>VRSFIYEPFQIPSGSMMPTLLIGDFILVEKFAYGIKDPIYQKTLIETGHPKRGDIVVFKYPEDPKLDYIKRAVGLPGDKVTYDPVSKELTIQPGCSSGQACENALPVTYSNVEPSDFVQTFSRRNGGEAT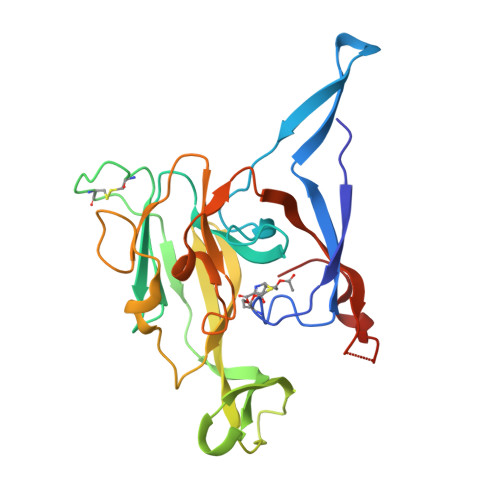SGFFEVPKNETKENGIRLSERKETLGDVTHRILTVPIAQDQVGMYYQQPGQQLATWIVPPGQYFMMGDNRDNSADSRYWGFVPEANLVGRATAIWMSFDKQEGEWPTGLRLSRIGGIH[4x]> GAMFQIKARPYERFADVEKPWIQKHSMDSKLVPANKGNLIQAEIVYQSVSEHSDLVISPVNEIRPANRFPSHRKSFFAENLRASPPVVPVAVDKYAVPVANPMDPENPNAWDVTLKITTKAVTVPVDVVMVIDQSSSMGGQNIARLKSAIASGQRFVKKMLPKGMATEGVRIALVSYDHEPHRLSDFTKDTAFLCQKIRALTPIWGTHTQGGLKMARNIMATSTAVDKHIILMSDGLATEQYPVKNVTTADFIGETGNANDPIDLVIQGAINFPTNYVSNNPSTPLTPNYPTHSSKVGRRNLPESKFDYSNLSARITFDGVAGALVYEPRFPHPYYYYFPCNAAINEAQFAKNSGYTIHTIGYDLGDFALANNSLKLTATDENHFFTATPANLAAAFDNIAQTINIGIQRGEVTDFVAPGFIVKNLTQSGDVTHLLNVSNGTVHYDVSTKKLTWTTGTILSSSEATITYRIYADLDYIQNNDIPVNTTSAIGPDLGGFDTNTEAKLTYTNSNGESNQQLIFPRPTVKLGYGVIKRHYVLVNKDGQPIQANGTVVSSLSEAHVLQSQDFFLPSGGGHIVPKWIKLDKTTEALQYYSVPPTNTVITTADGKRYRFVEVPGSTPNPGQIGISWKKPAGNAYFAYKLLNYWMGGTTDQQSEWDVTSNWTGAQVPLTGEDVEFATTENFGSPAVADLHVPTTNPKIIGNLINNSDKDLVVTTNSQLTINGVVEDNNPNVGTIVVKSSKDNPTGTLLFANPGYNQNVGGTVEFYNQGYDCADCGMYRRSWQYFGIPVNESGFPINDVGGNETVNQWVEPFNGDKWRPAPYAPDTKLQKFKGYQITNDVQAQPTGVYSFKGTLCVCDAFLNLTRTSGVNYSGANLIGNSYTGAIDIKQGIVFPPEVEQTVYLFNTGTRDQWRKLNGSTVSGFRAGQYLSVPKNTAGQDNLPDRIPSMHSFLVKMQNGASCTLQILYDKLLKNTTVNNGNGTQITWRSGNSGSANMPSLVMDVLGNESADRLWIFTDGGLSFGFD

P. gingivalis expresses two antigenically distinct but structurally homologous type-V fimbriae that are important both for attachment to other bacteria and for invasion of different host tissues. Instead, Mfa5 is the only fimbrial protein that has been found to be dependent on the type-IX secretion system for translocation across the outer membrane. Surprisingly, despite being unrelated in sequence, Mfa5 shows a striking similarity to the Gram-positive adhesins RrgA and GBS104, which both have a vWF domain and a number of IgG-like domains that appear to function as the stalk to project the VWF domain toward ligands, presumably those presented on host cells. Thus the vWF domain is a clear indication that the D1 domain of Mfa5 functions as an adhesin, but the ligand has yet not been determined.

In this study, we present the crystal structure of the N-terminal half of Mfa5, residues 99–664, at 1.8 Å resolution. The structure consists of three domains (D1 to D3) that build up an elongated shape with dimensions of 46 Å × 48 Å × 164 Å. The first domain, D1 (amino acids 142–418), forms a Rossman fold classified as a vWF domain. The vWF domain comprises a cleft harboring a MIDAS motif with a bound Mg2+ ion. The second domain, D2 (amino acids 105–135 and 423–544), has an IgG-like fold composed of a β-sandwich with three and five β-strands, respectively. Intriguingly, the vWF domain is inserted between strands B (first sheet) and C (second sheet) of the D2 domain. Interestingly, an intramolecular isopeptide bond connects Lys111 of the first β-sheet to Asn518 of the second β-sheet. Instead, the isopeptide bond is stabilized by Thr517 (OG) and by Tyr486 (OH) via a water molecule. D3, encompassing amino acids 547–664, comprises six β-strands in a twisted tube-like β-sheet that can be classified as a ubiquitin-like roll. The D3 domain folds like an incomplete IgG-like domain, and comparison to the IgG-like domains in RrgA and GBS104 lead us to speculate that strands are missing from this domain.During bacterial cell division, filaments of tubulin-like FtsZ form the Z-ring, which is the cytoplasmic scaffold for divisome assembly. In Escherichia coli, actin homologue FtsA anchors the Z-ring to the membrane and recruits divisome components, including bitopic FtsN. In E. coli and many other bacteria, FtsA is the main membrane anchor for the cell division ring, the Z-ring, which initiates and organises division.

We identified an FtsA-FtsN interaction site in FtsA’s IA-IC interdomain cleft by X-ray crystallography and confirmed that FtsA forms double filaments in vivo by site-specific cysteine cross-linking. The 16 FtsA monomers are organised into four tetramers, each containing two short antiparallel protofilaments comprising two FtsA monomers (Supplementary Movie M1). One of the two FtsA monomers in each protofilament adopts a closed and the other one an open conformation. The IC domain in the open conformation is rotated downwards by 13.8 ° compared to the closed conformation, as analysed by DynDom38. The IC domains in the lateral interfaces of each tetramer are twisted against each other compared to the straight VmFtsA1-396 double filament. Several hydrogen bonding contacts are lost because of the bending when compared to the straight filament (Figure 3a, asterisks). FtsN and PilN both bind in the IA-IC interdomain cleft (using FtsA domain nomenclature for PilM), but use different binding modes. FtsN binds further downward in the cleft, predominantly contacting the IC domain of FtsA. Importantly, our structural data reveal that the FtsA double filament is compatible with FtsN binding.

>MTKTTDDNIIVGLDIGTATVSALVGEVLPDGQVNIIGAGSSPSRGMDKGGVNDLESVVKSVQRAVDQAELMAECQISSVFISLSGKHIASRIEKGMGTISEEEVSQDDMDRAIHTAKSIKIGDEQRILHVIPQEFTIDYQEGIKNPLGLSGVRMEVSVHLISCHNDMARNIIKAVERCGLKVEQLVFSGLASSNAVITEDERELGVCVVDIGAGTMDISIWTGGALRHTEVFSYAGNAVTSDIAFAFGTPLSDAEEIKVKYGCALSELVSKDDTVNVPSVGGRPSRSLQRQTLAEVIEPRYTELMGLVNQTIDNVQAKLRENGVKHHLAAGVVLTGGAAQIEGVVECAERVFRNQVRVGKPLEVSGLTDYVKEPYHSTAVGLLHYARDSQDNDDND[16x]> MASDGVVVEIGKVTGSVGTTVEIPVYFRGVPSKGIANCDFVFRYDPNVLEIIGIDPGDIIVDPNPTKSFDTAIYPDRKIIVFLFAEDSGTGAYAITKDGVFAKIRATVKSSAPGYITFDEVGGFADNDLVEQKVSFIDGGVNVG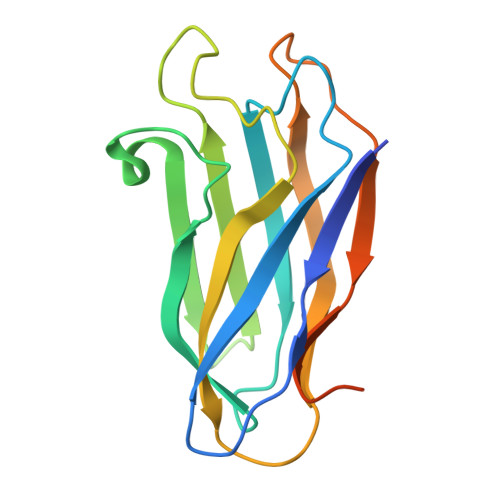NATPTKGATPTNTATPTK>[4x]KKIKLNIKEFKATAEGLSPEEKELWDKFAEKLKKELNNKIINLGEKIEIEEELKTPTKSIKITFSLELVSEDTFKATLKLEIKGKETIVEEETV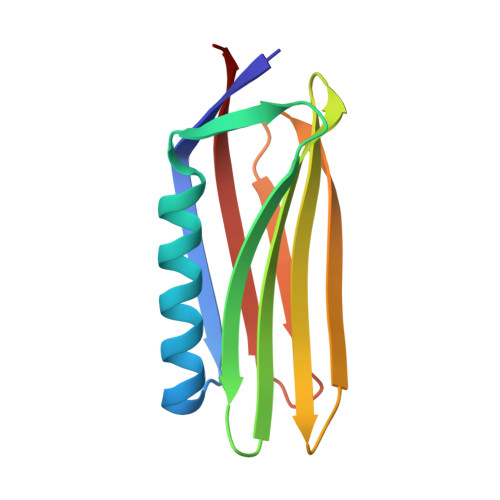EFKAGETVKLTIKLPDGKTFTLELKLEATKI>SSKEVAELKKQVESAELKNQRLKEVFQTKIQEFRKACYTLTGYQID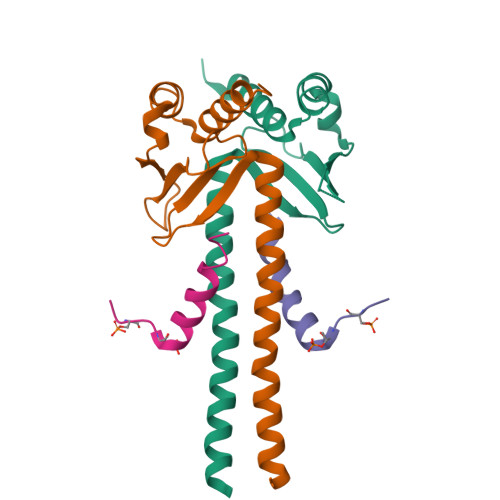ITTENQYRLTSLYAEHPGDCLIFKATSPSGSKMQLLETEFSHTVGELIEVHLRRQDSIPAFLSSLTLELFSRQTVA[2x];>[2x]KVQPSPTVHTKEALGFIMNMFQAPTS2-hydroxy-1-phenylethanone | 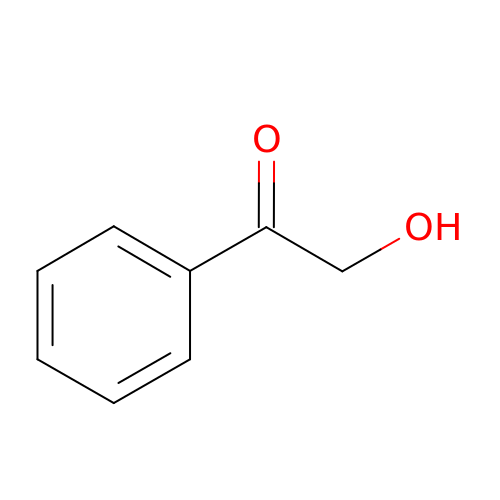C8 H8 O2 | ZWVHTXAYIKBMEE-UHFFFAOYSA-N>[4x]GAMGSEESLKHATRIIDEVVSKFLDDLGNAKSHLMS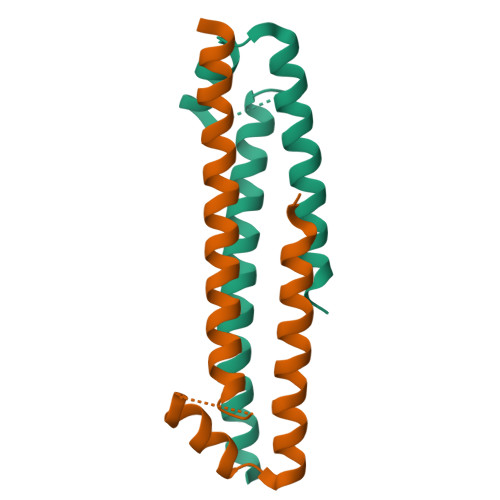LYSACSSEVPPGPVDQKFQSIVIGCALEDQKKIKRRLETLLRNIDNSDKAIK> GSHMATAVTARPGVPVTAAPPLRLASRNSVFTRSGAGPRYWNIYGYSFPHNAPIPENEWKVNIDWLAGNFADFGYDIACTDGWIEGSSRTTGNGYITSYNDSWQHDWAYWANYLAARKMKLGVYYNPLWVHRAAVEDASKTVLGRPDVKIADLVVPGDFFARDIGGNQLYWLDVTKSGAKEYVQGYVRYFKDLGVPYLRIDFLSWYEDGRDANIGQVNAPHGRANYELALSWINEAAGEDMEVSLVMPHMFQDGSAELANGDLVRINADADKGGWDRL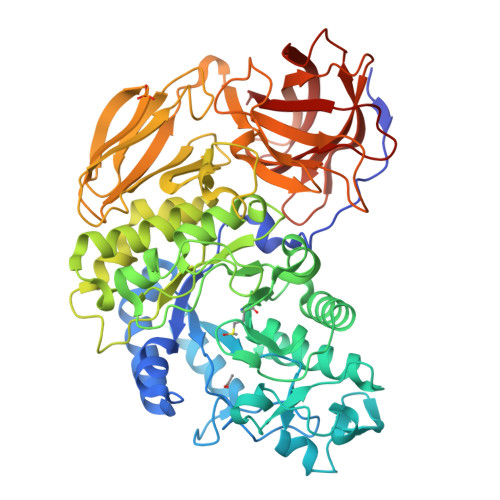SGMRQNWQDAWPNWANPFCGFTGWSHRNGRGQLILDGDFMRASTFASDEERKTMMNLMVAAGSPLAIADTYQQIGNNAWVYTNKEVLQLNADGLVGKPLYRSATPFSKDPGSRDTERWAGQLPDGSWGVALFNRSDTETVTKTIDFAKDLGLATGGNVRDLWEHRNLGMDSRATAALAPHASAIFRVTPPKMHGTTRYPAAFAAWGGGAGFNYNHPGYDGNGFVDGLQAGSGSADPLVTFAVQVPHRGSYAIRYRYANATGDTSTMTVTAEKADRSTVDGPVHVSFPGLATWDTWGVADGTITLDAGLNLVTIGRGATDKGAINLNWIELDM> VVSFIGSTENDVGPSQGSYSSTHAMDNLPFVYNTGYNIGYQNANVWRIGGGFCVGLDGKVDLPVVGSLDGQSIYGLTEEVGLLIWMGDTNYSRGTAMSGNSWENVFSGWSVGNYLS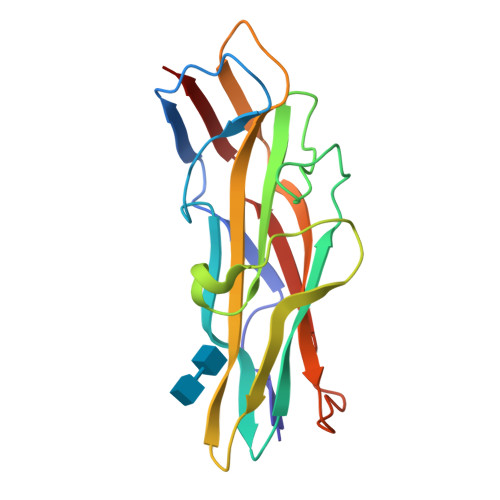TQGLSVHVRPVILKRNSSAQYSVQKTSIGSIRMRPYNGSSAGSVQTTVNFSLNPFTLNDT>GPSGHSARKKPLLQNRHKKARLRFATAHGDKDRTFWRNVLWSDETKIELFGHNDHRYVWRKKGEACKPKNTIPTVKHGGGSIMLWGCFAAGGTGALHKIDGIMDAVQYVDILKQHLKTSVRKLKLGRKWVFQHDNDPKHTSKVVAKWLKDNKVKVLEWPSQSPDLNPIENLWAELKKRVRARRPTNLTQLHQLCQEEWAKIHPNYCGKLVEGYPKRLTQVKQFKGNATKY[2x]

SB is a member of the widespread Tc1/mariner superfamily of DNA transposons that has been developed as a genome engineering tool in a broad range of organisms. The transposon (tnp) DNA includes terminal inverted repeats (TIRs) at its ends and encodes a transposase protein, the workhorse of transposition, that catalyses all DNA cleavage and joining reactions required for transposition. Tc1/mariner transposases contain an N-terminal bipartite PAIRED-like10 DNA-binding domain (DBD) consisting of two helix-turn-helix motifs, and a C-terminal catalytic domain with an RNaseH-like fold and a catalytic triad of three acidic residues (DDE)1 that execute DNA hydrolysis (in excision) and transesterification (in integration) in a two metal ion-dependent manner. The 39 kDa SB transposase (340 amino acids (aa)) features a similar domain composition to other Tc1/mariner transposases.

To provide structural insights into SB transposition, we crystallized the catalytic domain (aa 114–340; including most of the flexible inter-domain linker that spans aa 110–127) of the current most active SB transposase variant2, SB100X, and solved its structure at 1.4 Å resolution. The core of the structure reveals a canonical RNaseH-fold, consisting of a central five-stranded β-sheet (β1–β5) surrounded by five α-helices (α1–α5). The catalytic residues (D153, D244 and E279) are assembled in close proximity establishing an active site conformation similar to the one observed in the crystal structure of the homologous Mos1 transposase PEC (grey in Figs 1a,b). In addition to the core RNaseH domain, most of the inter-domain linker (aa 117–127) and also the flexible clamp loop (aa 159–190), which is inserted between β1 and β2 of the RNaseH-fold7 and includes part of the glycine-rich strip (aa 183–190), are visible in the structure. In the Mos1 PEC, the clamp loop is extended and interacts with the similarly extended linker and both tnp ends across the dimer interface, playing an important role in PEC assembly. In turn, in our SB100X catalytic domain crystals, the clamp loop is curved, mostly pivoting on three consecutive G-s (aa 188–190, marked with red arrow in Fig. 1a) in the glycine-rich strip, and contributes to an extended protein–protein interface (2,350 Å2 surface area; ΔG=−27.2 kcal mol−1)29 between symmetry related molecules in neighbouring asymmetric units. The clamp loops of both protomers form reciprocal interactions with the RNaseH core of the partner molecule, covering the active sites. In addition, the tip of the clamp loop contains two short antiparallel β-strands (aa 169–171 and 174–176), which form a β-hairpin and interact with the main chain of the inter-domain linker (aa 119–122) of the partner molecule. However, as the observed arrangement of the catalytic domains is too compact to allow DNA to access the active sites, it does not appear compatible with PEC assembly.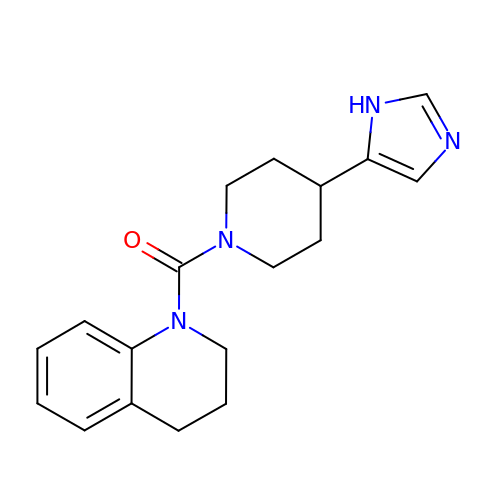3,4-dihydroquinolin-1(2H)-yl[4-(1H-imidazol-5-yl)piperidin-1-yl]methanone | C18 H22 N4 O | UTSIHHDNMUZNMG-UHFFFAOYSA-N> IVGGQECKDGECPWQALLINEENEGFCGGTILSEFYILTAAHCL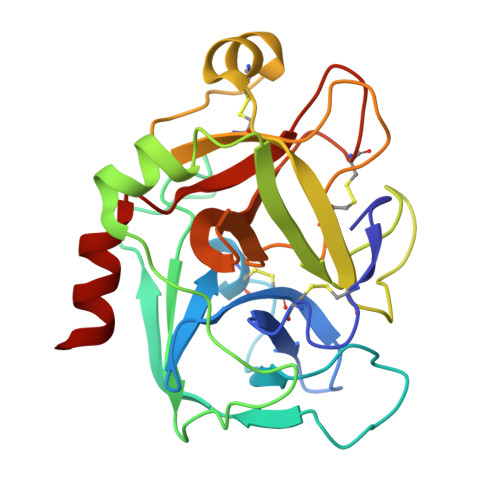YQAKRFKVRVGDRNTEQEEGGEAVHEVEVVIKHNRFTKETYDFDIAVLRLKTPITFRMNVAPACLPERDWAESTLMTQKTGIVSGFGRTHEKGRQSTRLKMLEVPYVDRNSCKLSSSFIITQNMFCAGYDTKQEDACQGDSGGPHVTRFKDTYFVTGIVSWGEGCARKGKYGIYTKVTAFLKWIDRSMKT> MHHGTGPQNVQHQL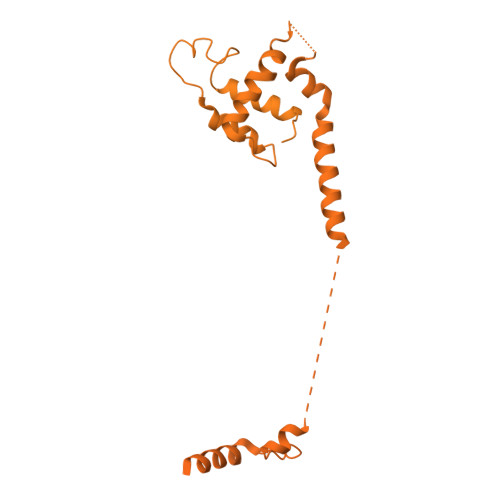QRSRACPGSEGEEQPAHPNPPPSPAAPFAPSASPSAPQSPSYQIQQLMNRSPATGQNVNITLQSVGPVVGGNQQITLAPLPLPSPTSPGFQFSAQPRRFEHGSPSYIQVTSPLSQQVQTQSPTQPSPGPGQALQNVRAGAPGPGLGLCSSSPTGGFVDASVLVRQISLSPSSGGHFVFQDGSGLTQIAQGAQVQLQHPGTPITVRERRPSQPHTQSGGTIHHLGPQSPAAAGGAGLQPLASPSHITTANLPPQISSIIQGQLVQQQQVLQGPPLPRPLGFERTPGVLLPGAGGAAGFGMTSPPPPTSPSRTAVPPGLSSLPLTSVGNTGMKKVPKKLEEIPPASPEMAQMRKQCLDYHYQEMQALKEVFKEYLIELFFLQHFQGNMMDFLAFKKKHYAPLQAYLRQNDLDIEEEEEEEEEEEEKSEVINDEVKVVTGKDGQTGTPVAIATQLPPKVSAAFSSQQQPFQQALAGSLVAGAGSTVETDLFKRQQAMPSTGMAEQSKRPRLEVGHQGVVFQHPGADAGVPLQQLMPTAQGGMPPTPQAAQLAGQRQSQQQYDPSTGPPVQNAASLHTPLPQLPGRLPPAGVPTAALSSALQFAQQPQVVEAQTQLQIPVKTQQPNVPIPAPPSSQLPIPPSQPAQLALHVPTPGKVQVQASQLSSLPQMVASTRLPVDPAPPCPRPLPTSSTSSLAPVSGSGPGPSPARSSPVNRPSSATNKALSPVTSRTPGVVASAPTKPQSPAQNATSSQDSSQDTLTEQITLENQVHQRIAELRKAGLWSQRRLPKLQEAPRPKSHWDYLLEEMQWMATDFAQERRWKVAAAKKLVRTVVRHHEEKQLREERGKKEEQSRLRRIAASTAREIECFWSNIEQVVEIKLRVELEEKRKKALNLQKVSRRGKELRPKGFDALQESSLDSGMSGRKRKASISLTDDEVDDEEETIEEEEANEGVVDHQTELSNLAKEAELPLLDLMKLYEGAFLPSSQWPRPKPDGEDTSGEEDADDCPGDRESRKDLVLIDSLFIMDQFKAAERMNIGKPNAKDIADVTAVAEAILPKGSARVTTSVKFNAPSLLYGALRDYQKIGLDWLAKLYRKNLNGILADEAGLGKTVQIIAFFAHLACNEGNWGPHLVVVRSCNILKWELELKRWCPGLKILSYIGSHRELKAKRQEWAEPNSFHVCITSYTQFFRGLTAFTRVRWKCLVIDEMQRVKGMTERHWEAVFTLQSQQRLLLIDSPLHNTFLELWTMVHFLVPGISRPYLSSPLRAPSEESQDYYHKVVIRLHRVTQPFILRRTKRDVEKQLTKKYEHVLKCRLSNRQKALYEDVILQPGTQEALKSGHFVNVLSILVRLQRICNHPGLVEPRHPGSSYVAGPLEYPSASLILKALERDFWKEADLSMFDLIGLENKITRHEAELLSKKKIPRKLMEEISTSAAPAARPAAAKLKASRLFQPVQYGQKPEGRTVAFPSTHPPRTAAPTTASAAPQGPLRGRPPIATFSANPEAKAAAAPFQTSQASASAPRHQPASASSTAASPAHPAKLRAQTTAQASTPGQPPPQPQAPSHAAGQSALPQRLVLPSQAQARLPSGEVVKIAQLASITGPQSRVAQPETPVTLQFQGSKFTLSHSQLRQLTAGQPLQLQGSVLQIVSAPGQPYLRAPGPVVMQTVSQAGAVHGALGSKPPAGGPSPAPLTPQVGVPGRVAVNALAVGEPGTASKPASPIGGPTQEEKTRLLKERLDQIYLVNERRCSQAPVYGRDLLRICALPSHGRVQWRGSLDGRRGKEAGPAHSYTSSSESPSELMLTLCRCGESLQDVIDRVAFVIPPVVAAPPSLRVPRPPPLYSHRMRILRQGLREHAAPYFQQLRQTTAPRLLQFPELRLVQFDSGKLEALAILLQKLKSEGRRVLILSQMILMLDILEMFLNFHYLTYVRIDENASSEQRQELMRSFNRDRRIFCAILSTHSRTTGINLVEADTVVFYDNDLNPVMDAKAQEWCDRIGRCKDIHIYRLVSGNSIEEKLLKNGTKDLIREVAAQGNDYSMAFLTQRTIQELFEVYSPMDDAGFPVKAEEFVVLSQEPSVTETIAPKIARPFIEALKSIEYLEEDAQKSAQEGVLGPHTDALSSDSENMPCDEEPSQLEELADFMEQLTPIEKYALNYLELFHTSIEQEKERNSEDAVMTAVRAWEFWNLKTLQEREARLRLEQEEAELLTYTREDAYSMEYVYEDVDGQTEVMPLWTPPTPPQDDSDIYLDSVMCLMYEATPIPEAKLPPVYVRKERKRHKTDPSAAGRKKKQRHGEAVVPPRSLFDRATPGLLKIRREGKEQKKNILLKQQVPFAKPLPTFAKPTAEPGQDNPEWLISEDWALLQAVKQLLELPLNLTIVSPAHTPNWDLVSDVVNSCSRIYRSSKQCRNRYENVIIPREEGKSKNNRPLRTSQIYAQDENATHTQLYTSHFDLMKMTAGKRSPPIKPLLGMNPFQKNPKHASVLAESGINYDKPLPPIQVASLRAERIAKEKKALADQQKAQQPAVAQPPPPQPQPPPPPQQPPPPLPQPQAAGSQPPAGPPAVQPQPQPQPQTQPQPVQAPAKAQPAITTGGSAAVLAGTIKTSVTGTSMPTGAVSGNVIVNTIAGVPAATFQSINKRLASPVAPGALTTPGGSAPAQVVHTQPPPRAVGSPATATPDLVSMATTQGVRAVTSVTASAVVTTNLTPVQTPARSLVPQVSQATGVQLPGKTITPAHFQLLRQQQQQQQQQQQQQQQQQQQQQQQQQQQQQTTTTSQVQVPQIQGQAQSPAQIKAVGKLTPEHLIKMQKQKLQMPPQPPPPQAQSAPPQPTAQVQVQTSQPPQQQSPQLTTVTAPRPGALLTGTTVANLQVARLTRVPTSQLQAQGQMQTQAPQPAQVALAKPPVVSVPAAVVSSPGVTTLPMNVAGISVAIGQPQKAAGQTVVAQPVHMQQLLKLKQQAVQQQKAIQPQAAQGPAAVQQKITAQQITTPGAQQKVAYAAQPALKTQFLTTPISQAQKLAGAQQVQTQIQVAKLPQVVQQQTPVASIQQVASASQQASPQTVALTQATAAGQQVQMIPAVTATAQVVQQKLIQQQVVTTASAPLQTPGAPNPAQVPASSDSPSQQPKLQMRVPAVRLKTPTKPPCQ> MTGGLVLNAISRAGGAMGGLGLIKSLAEKEKQLLERLEAAKKEAEERVKRAEAEAKALLEEAEAKAKALEAQYRERERAETEALLARYRERAEAEAKAVREKAMARLDEAVALVLKEVLP;> MSKLEAILSQEVEAEIQALLQEAEAKAEAVKREAEEKAKALLQARERALEAQYRAALRRAESAGELLVATARTQARGEVLEEVRRRVREALEALPQKPEWPEVVRKLALEALEALPGAKALVANPEDLPHLEALARERGVELQAEPALRLGVRAVGAEGKTQVENSLLARLDRAWDALSSKVAQALWG;> MADDFAYLNARVRVRRGTLLKESFFQEALDLSFADFLRLLSETVYGGELAGQGLPDVDRAVLRTQAKLVGDLPRLVTGEAREAVRLLLLRNDLHNLQALLRAKATGRPFEEVLLLPGTLREEVWRQAYEAQDPAGMAQVLAVPGHPLARALRAVLRETQDLARVEALLAKRFFEDVAKAAKGLDQPALRDYLALEVDAENLRTAFKLQGSGLAPDAFFLKGGRFVDRVRFARLMEGDYAVLDELSGTPFSGLSGVRDLKALERGLRCVLLKEAKKGVQDPLGVGLVLAYVKEREWEAVRLRLLARRAYFGLPRAQVEEEVVCP;> MIAPMEKLVLAGPKGRAKELLQSLQQAGVVHLETLRPEALSAYQLSPEERAELRRWEAVSAGAEHTLSLLGLEAEPARPFPEGLEAAEKALSPIQAHAEGLTRQKQELEEELALAQAYLEPLERLAALAHGLDKSPFLRVIPFLLTEKELPLVEEALRKALEDRYLLAHEAYAGGVAALVVVHRKEVDQAKAALSRAGVAELRLPGALGELPLSEAARR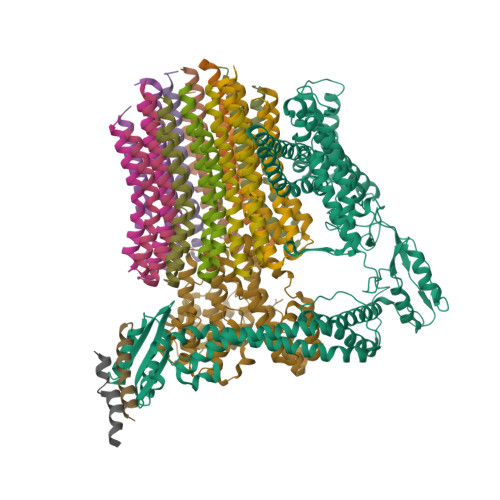LKERAEAAPRELSEVRQHLAKLARESASTLQSLWTRAQDEVARLKALEELASGRFGFALLGYVPVKAKPKVEEALARHKESVVYAFEPVDEHHEADRIPVVLDNPPWAKPFELLVSFLNTPKYGTFDPTPVVPVFFPFWFGMIVGDIGYALLFYLVGRWLSGYVKRNEPLVIDLFALKLKPQVIGKLVHILNWMVFWTVVWGVIYGEFFGTFLEHLGVFGTPEHPGLIPILIHRIDTAKTANLLILLSVAFGVVLVFFGLALRAYLGLKHRHMAHFWEGVGYLGGLVGVLALAASYLGNLQAGWLQGLMYLGFGVFLLAVLMSRIWLMIPEIFTQAGHILSHIRIYAVGAAGGILAGLLTDVGFALAERLGLLGVLLGLLVAGVLHLLILLLTTLGHMLQPIRLLWVEFFTKFGFYEENGRPYRPFKSVREAQ;>[12x]MKKLLVTVLLAVFGALAFAAEEAAASGGLDRGLIAVGMGLAVGLAALGTGVAQARIGAAGVGAIAEDRSNFGTALIFLLLPETLVIFGLLIAFILNGRLHHH> MAVKVEYDLKRLRNIGIAAHIDAGKTTTTERILYYTGRIHKIGEVHEGAATMDFMEQERERGITITAAVTTCFWKDHRINIIDTPGHVDFTIEVERSMRVLDGAIVVFDSSQGVEPQSETVWRQAEKYKVPRIAFANKMDKTGADLWLVIRTMQERLGARPVVMQLPIGREDTFSGIIDVLRMKAYTYGNDLGTDIREIPIPEEYLDQAREYHEKLVEVAADFDENIMLKYLEGEEPTEEELVAAIRKGTIDLKITPVFLGSALKNKGVQLLLDAVVDYLPSPLDIPPIKGTTPEGEVVEIHPDPNGPLAALAFKIMADPYVGRLTFIRVYSGTLTSGSYVYNTTKGRKERVARLLRMHANHREEVEELKAGDLGAVVGLKETITGDTLVGE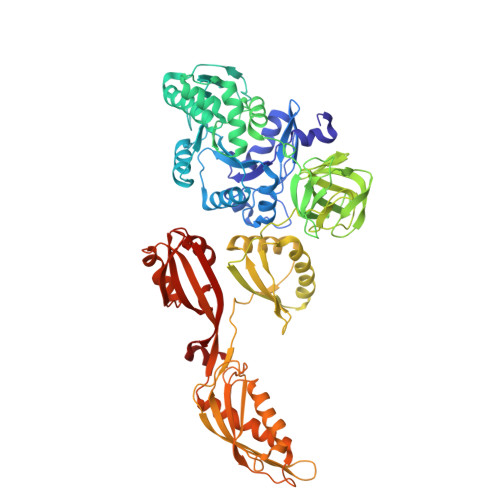DAPRVILESIEVPEPVIDVAIEPKTKADQEKLSQALARLAEEDPTFRVSTHPETGQTIISGMGELHLEIIVDRLKREFKVDANVGKPQVAYRETITKPVDVEGKFIRQTGGRGQYGHVKIKVEPLPRGSGFEFVNAIVGGVIPKEYIPAVQKGIEEAMQSGPLIGFPVVDIKVTLYDGSYAEVDSSEMAFKIAGSMAIKEAVQKGDPVILEPIMRVEVTTPEEYMGDVIGDLNARRGQILGMEPRGNAQVIRAFVPLAEMFGYATDLRSKTQGRGSFVMFFDHYQEVPKQVQEKLI> MANKDG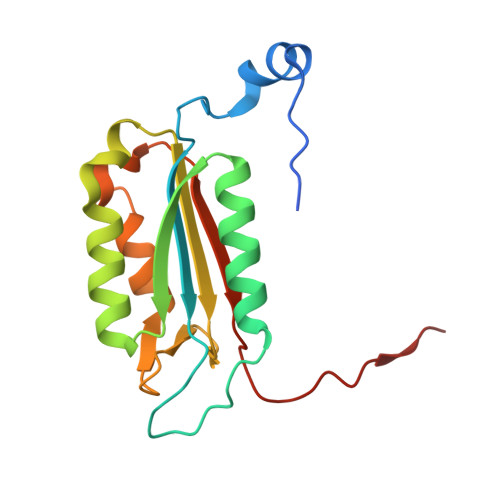PVCLQVKPCTPEFYQTHFQLAYRLQSRPRGLALVLSNVHFTGEKELEFRSGGDVDHSTLVTLFKLLGYDVHVLCDQTAQEMQEKLQNFAQLPAHRVTDSCIVALLSHGVEGAIYGVDGKLLQLQEVFQLFDNANCPSLQNKPKMFFIQACRGDETDRGVDQQD> AKA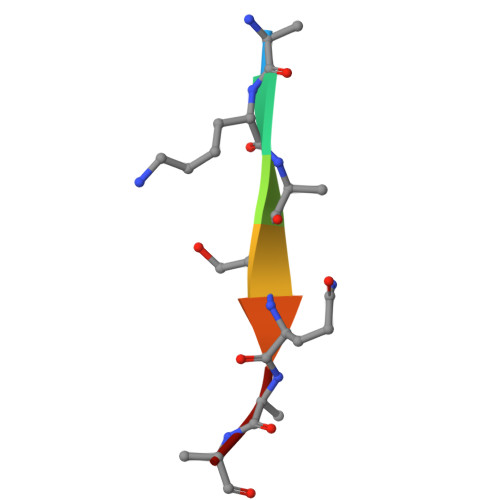SQAA Intersectin-1L is a large (∼190 kDa), modular, endocytic scaffolding protein that also has GEF activity for Cdc42. It is composed of two N-terminal Eps15-homology (EH) domains, a putative coiled-coiled domain, five SH3 domains related with a sequence identity of 30%–40% (SH3 A, B, C, D, E), followed by the DH and PH domains and a carboxyl-terminal C2 domain. A number of studies have addressed the pathways downstream of the intersectin-1L GEF activity, which is highly specific for the Rho GTPase Cdc42. The intersectin-1L SH3 domains negatively regulate the in vitro GEF activity of the adjacent DH domain.

We were unable to crystallize the SH3(E)-DH-PH fragment, but the SH3(E)-DH fragment (1151–1431) yielded well-formed, hexagonal-shaped crystals, belonging to space group P3221 with two chains in the asymmetric unit. The SH3(E) domain in one of the two protein chains is disordered and thus was not modeled. The linker connecting the SH3(E) domain and DH domain (1204–1225) is well ordered in both chains of the asymmetric unit, with residues 1210–1214 unexpectedly forming a short α-helix. The DH domain (1226–1431) is an elongated helical bundle structurally homologous to other DH domains of known structure. The GEF activity of intersectin-1L is controlled by a core autoinhibitory interaction involving the fifth SH3 domain (SH3(E)) and the catalytic DH domain The crystal structure of the SH3(E)-DH domain fragment presented here reveals a homodimer in a domain swapped arrangement with the SH3 from one monomer forming an intermolecular interaction with the DH domain of the other monomer. The SH3(E) domain from one monomer forms an intermolecular interaction with the C-terminal half of the DH domain from the second monomer. This interaction occurs side of the DH-domain opposite the Cdc42 GTPase binding site. It buries 534 Å2 of surface area on the DH domain, and involves contacts with the first half of α2, the middle fragment of α3, and one face of the c-terminal region of α6 (with the other face of α6 interacting with the DH domain from the other chain). The structure of the “repressed” DH domain as reported in this study is highly similar to the “active” DH domain observed in the crystal structure of human intersectin-1L complexed with Cdc42. However, both analytical ultracentrifugation and gel filtration analysis indicate the nucleotide exchange repressed SH3(E)-DH fragment is exclusively monomeric at micromolar concentrations, more than 100 times greater than used in the in vitro nucleotide exchange activity assay.

>GSCQVIGMYDYTAQNDDELAFSKGQIINVLNKEDPDWWKGEVSGQVGLFPSNYVKLTTDMDPSQQWCSDLHLLDMLTPTERKRQGYIHELIVTEENYVNDLQLVTEIFQKPLTESELLTEKEVAMIFVNWKELIMCNIKLLKALRVRKKMSGEKMPVKMIGDILSAQLPHMQPYIRFCSCQLNGAALIQQKTDEAPDFKEFVKRLAMDPRCKGMPLSSFILKPMQRVTRYPLIIKNILENTPENHPDHSHLKHALEKAEELCSQVNEGVREKENSDRLEWIQA[2x]> MGWSCIILFLVATATGVHSNPPTFSPALLVVTEGDSATFTCSFSSTSESFVLNWYRMSPSGQPDKLAAFPEDRSQPGQDSRFRVTQLPNGRDFHMSVVRARRDDSGTYLCGAISLAPK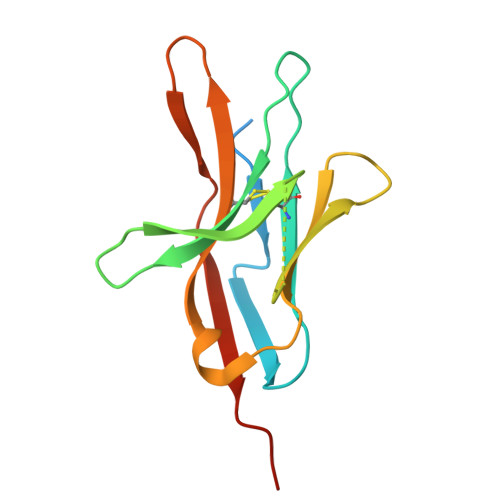VQIKESLRAELRVTERRAEPEA> GDDDDDNGGSSVMNITGIYLEDAKSNVPDRLVDFARLGQLIRIEGEGFNGLKKVYINGYNCYFNPVFVSNKSFLVSVNSKVPTTEADENVRNTIRLVKDGGEYVYDFQIRAAAPSITKISNCMPNVGEPIIVYGSGLTEIAKVVFPGNVVVTEGIISDLDGEYFMVDMPAGVSEEGGSIFVEGSNGGAYSPAYFNYKKGLLLNFDGVGAQGAWGDSESMIQTTELESASIGEGNVSQGAYCRLPLERQLPVAAAKNR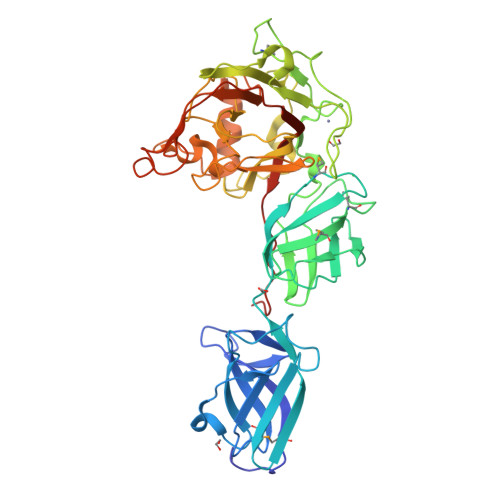CAEVWTAGNGTDPDWLTLGVPAETPVAECAIQFEIYVPEPWSESGFLKICGQNGFNGGEWERDCYNYVPWLVDGKIVPFQTTGWQTVTVPFSEFYKSKASSGAWTTFADVTATRASASYANFGFYFENSDITLDKITGASSDKETEFLSKATSVKIYIDNWRVVPLTKPEYTDFPDEEEDAE Montbretin A 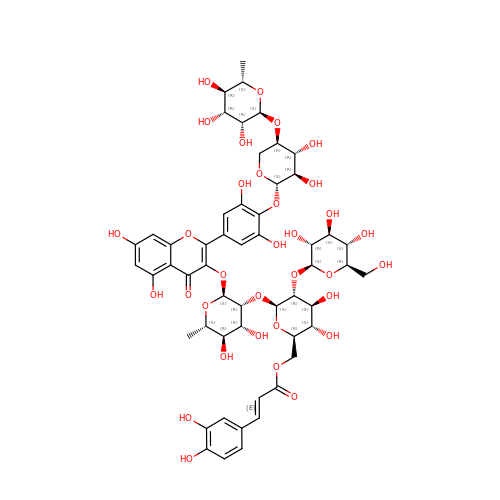| C53 H64 O33 | FHVDXUPJFGRQLV-OWPXYNISSA-N> MWSHPQFEKENLYFQGGMS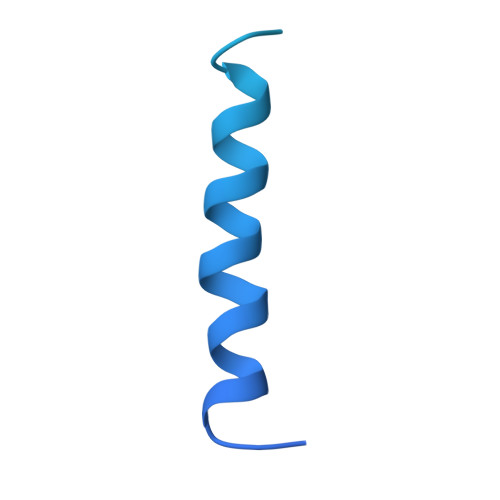KARRWVIIVLSLAVLVMIGINMAEKDDTAQVVVNNNDPTYKSEHTDTLVYNPEGALSYRLIAQHVEYYSDQAVSWFTQPVLTTFDKDKIPTWSVKADKAKLTNDRMLYLYGHVEVNALVPDSQLRRITTDNAQINLVTQDVTSEDLVTLYGTTFNSSGLKMRGNLRSKNAELIEKVRTSYEIQNKQTQP> QYAPQTQSGRTSIVHLFEWRWVDIALECERYLGPKGFGGVQVSPPNENVVVTNPSRPWWERYQPVSYKLCTRSGNENEFRDMVTRCNNVGVRIYVDAVINHMCGSGAAAGTGTTCGSYCNPGSREFPAVPYSAWDFNDGKCKTASGGIESYNDPYQVRDCQLVGLLDLALEKDYVRSMIADYLNKLIDIGVAGFRIDASKHMWPGDIKAVLDKLHNLNTNWFPAGSRPFIFQEVIDLGGEAIQSSEYFGNGRVTEFKYGAKLGTVVRKWSGEKMSYLKNWGEGWGFMPSDRALVFVDNHDNQRGHGAGGASILTFWDARLYKVAVGFMLAHPYGFTRVMSSYRWARNFVNGEDVNDWIGPPNNNGVIKEVTINADTTCGNDWVCEHRWREIRNMVWFRNVVDGQPFANW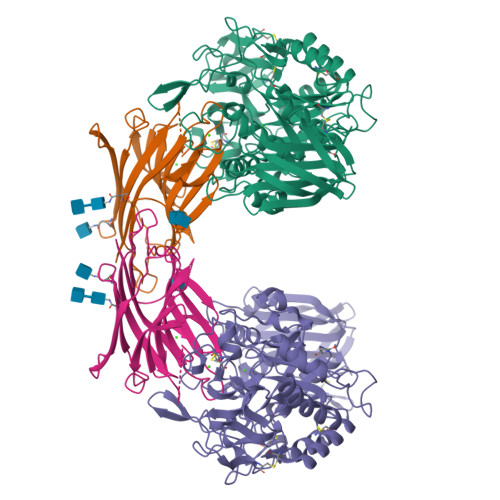WDNGSNQVAFGRGNRGFIVFNNDDWQLSSTLQTGLPGGTYCDVISGDKVGNSCTGIKVYVSSDGTAQFSISNSAEDPFIAIHAESKL;> ATETSFIIDAFNKTNLILQGDATVSSNGNLQLSYNSYDSMSRAFYSAPIQIRDSTTGNVASFDTNFTMNIRTHRQANSAVGLDFVLVPVQPESKGDTVTVEFDTFLSRISIDVNNNDIKSVPWDVHDYDGQNAEVRITYNSSTKVFSVSLSNPSTGKSNNVSTTVELEKEVYDWVSVGFSATSGAYQWSYETHDVLSWSFSSKFINLKDQKSERSNIVLNKIL(5S)-5-methyl-1-(quinolin-4-ylmethyl)-3-{4-[(trifluoromethyl)sulfonyl]phenyl}imidazolidine-2,4-dione 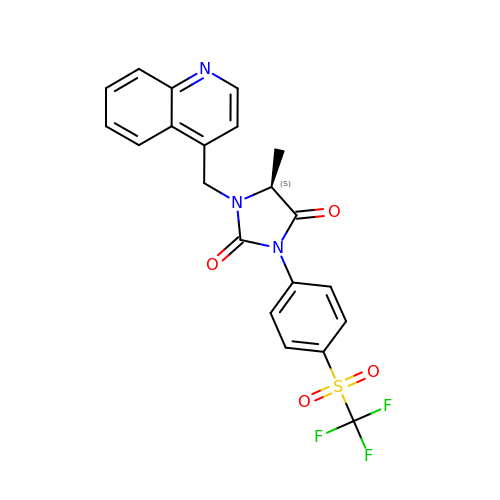| C21 H16 F3 N3 O4 S | GKQIKYWYJQQLLD-ZDUSSCGKSA-N> MSFINYSSREINCKIVYYGPGLCGKTTNLQYIYNKTAAETKGKLISLSTETDRTLFFDFLPLSLGEIRGFKTRFHLYTVPGQVFYDASRKLILKGVDGVVFVADSQIERMEANME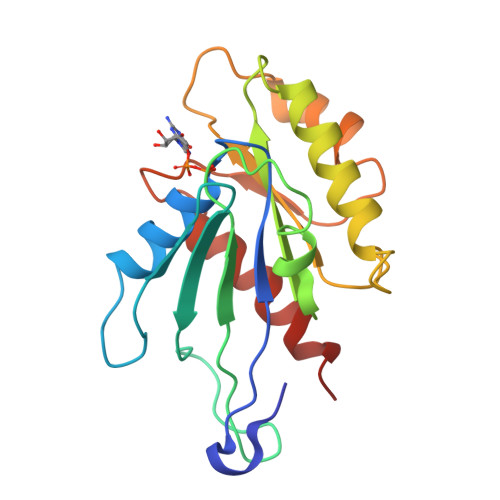SLENLRINLAEQGYDLNKIPYVIQYNKRDLPNAVTVEEMRKALNHRNIPEYQAVAPTGVGVFDTLKAVAKLVLTELKKGG> MMEYKIVENGLTYRIGNGASVPISNTGELIKGLRNYGPYEVPSLKYNQIALIHNNQFSSLINQLKSQISSKIDEVWHIHNINISEFIYDSPHFDSIKSQVDNAIDTGVDGIMLVLPEYNTPLYYKLKSYLINSIPSQFMRYDILSNRNLTFYVDNLLVQFVSKLGGKPWILNVDPEKGSDIIIGTGATRIDNVNLFCFAMVFKKDGTMLWNEISPIVTSSEYLTYLKSTIKKVVYGFKKSNPDWDVEKLTLHVSGKRPKMKDGETKILKETVEELKKQEMVSRDVKYAILHLNETHPFWVMGDPNNRFHPYEGTKVKLSSKRYLLTLLQPYLKRNGLEMVTPIKPLSVEIVSDNWTSEEYYHNVHEILDEIYYLSKMNWRGFRSRNLPVTVNYPKLVAGIIANVNRYGGYPINPEGNRSLQTNPWFL;> MGGSHHHHHHGMASENLYFQGGGGEIPLSSGNVNTPDVRSSGILYINIYPIVNYPETIKVSAIPYYEEFLPGKWKKRIGDLIYLY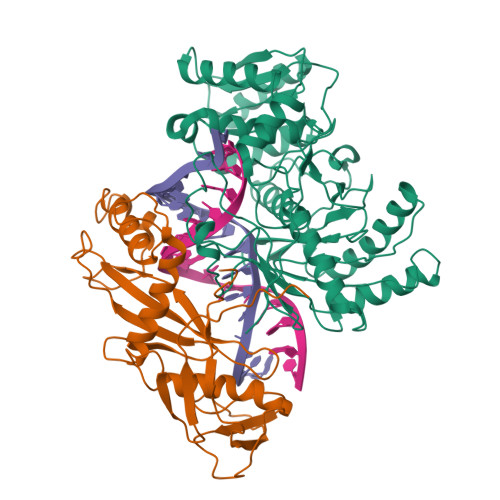GYGIENEFDEIDNSNALFGKIFRKYLLDILSENIATPWQLKELGSTLRLVKEITENYEFSNIIKLQYELIINVHHWQNTNFGIIVDLKINILDRENNQRISYTKIKDKYGESVKKKIWVSVQAFHRHLTPEGKKYATAMRDKFNLLTGLLKEAFGSSEDEKTFSTPDGEIKIVFKPLEIVEVSNNDGI6-hydroxy-2-methyl[1,3]thiazolo[4,5-d]pyrimidine-5,7(4H,6H)-dione 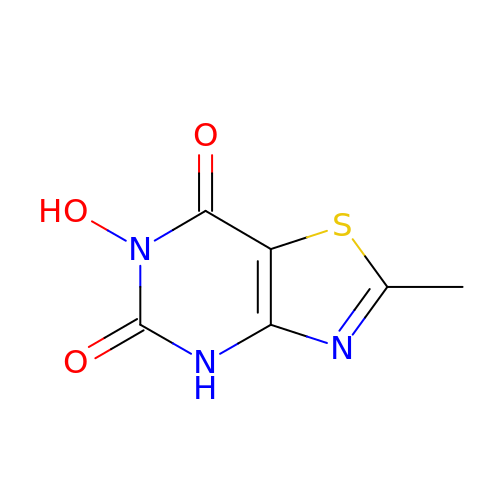| C6 H5 N3 O3 S | MYPICMPDMGFOBX-UHFFFAOYSA-N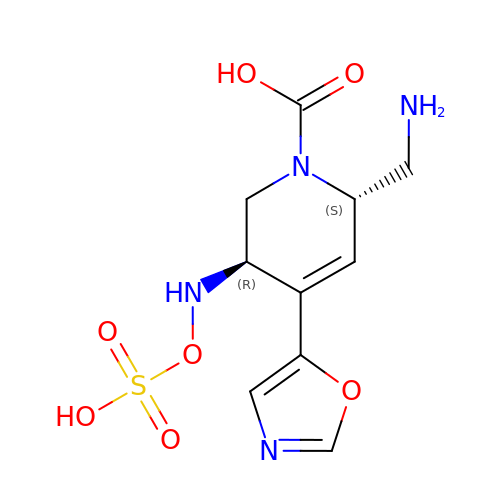(3~{R},6~{S})-6-(aminomethyl)-4-(1,3-oxazol-5-yl)-3-(sulfooxyamino)-3,6-dihydro-2~{H}-pyridine-1-carboxylic acid | C10 H14 N4 O7 S | ABKLGTMGWHFUKR-XPUUQOCRSA-N>MVKLAEFSRTATFAWSHDKIPLLVSGTVSGTVDANFSTDSSLELWSLLAADSEKPIASLQVDSKFNDLDWSHNNKIIAGALDNGSLELYSTNEANNAINSMARFSNHSSSVKTVKFNAKQDNVLASGGNNGEIFIWDMNKCTESPSNYTPLTPGQSMSSVDEVISLAWNQSLAHVFASAGSSNFASIWDLKAKKEVIHLSYTSPNSGIKQQLSVVEWHPKNSTRVATATGSDNDPSILIWDLRNANTPLQTLNQGHQKGILSLDWCHQDEHLLLSSGRDNTVLLWNPESAEQLSQFPARGNWCFKTKFAPEAPDLFACASFDNKIEVQTLQNLTNTLDEQETETKQQESETDFWNNVSREESKEKPSVFHLQAPTWYGEPSPAAHWAFGGKLVQITPDGKGVSITNPKISGLESNTTLSEALKTKDFKPLINQRLVKVIDDVNEEDWNLLEKLSMDGTEEFLKEALAFDNDESDAQDDANNEKEDDGEEFFQQIETNFQPEGDFSLSGNIEQTISKNLVSGNIKSAVKNSLENDLLMEAMVIALDSNNERLKESVKNAYFAKYGSKSSLSRILYSISKREVDDLVENLDVSQWKFISKAIQNLYPNDIAQRNEMLIKLGDRLKENGHRQDSLTLYLAAGSLDKVASIWLSEFPDLEDKLKKDNKTIYEAHSECLTEFIERFTVFSNFINGSSTINNEQLIAKFLEFINLTTSTGNFELATEFLNSLPSDNEEVKTEKARVLIASGKSLPAQNPATATTSKAKYTNAKTNKNVPVLPTPGMPSTTSIPSMQAPFYGMTPGASANALPPKPYVPATTTSAPVHTEGKYAPPSQPSMASPFVNKTNSSTRLNSFAPPPNPYATATVPATNVSTTSIPQNTFAPIQPGMPIMGDYNAQSSSIPSQPPINAVSGQTPHLNRKANDGWNDLPLKVKEKPSRAKAVSVAPPNILSTPTPLNGIPANAASTMPPPPLSRAPSSVSMVSPPPLHKNSRVPSLVATSESPRASISNPYAPPQSSQQFPIGTISTANQTSNTAQVASSNPYAPPPQQRVATPLSGGVPPAPLPKASNPYAPTATTQPNGSSYPPTGPYTNNHTMTSPPPVFNKPPTGPPPISMKKRSNKLASIEQNPSQGATYPPTLSSSASPLQPSQPPTLASQVNTSAENVSHEIPADQQPIVDFLKEELARVTPLTPKEYSKQLKDCDKRLKILFYHLEKQDLLTQPTIDCLHDLVALMKEKKYKEAMVIHANIATNHAQEGGNWLTGVKRLIGIAEATLN[2x];> MVVIANAHNELIHDAVLDYYGKRLATCSSDKTIKIFEVEGETHKLIDTLTGHEGPVWRVDWAHPKFGTILASCSYDGKVLIWKEENGRWSQIAVHAVHSASVNSVQWAPHEYGPLLLVASSDGKVSVVEFKENGTTSPIIIDAHAIGVNSASWAPATIEEDGEHNGTKESRKFVTGGADNLVKIWKYNSDAQTYVLESTLEGHSDWVRDVAWSPTVLLRSYLASVSQDRTCIIWTQDNEQGPWKKTLLKEEKFPDVLWRASWSLSGNVLALSGGDNKVTLWKENLEGKWEPAGEVHQ;> MVVIANAHNEMIHDAVMDYYGKRMATCSSDKTIKIFEVEGETHKLIDTLTGHEGPVWRVDWAHPKFGTILASCSYDGKVMIWKEENGRWSQIAVHAVHSASVNSVQWAPHEYGPMLLVASSDGKVSVVEFKENGTTSPIIIDAHAIGVNSASWAPATIEEDGEHNGTKESRKFVTGGADNLVKIWKYNSDAQTYVLESTLEGHSDWVRDVAWSPTVLLRSYMASVSQDRTCIIWTQDNEQGPWKKTLLKEEKFPDVLWRASWSLSGNVLALSGGDNKVTLWKENLEGKWEPAGEVHQ

COPII mediates Endoplasmic Reticulum to Golgi trafficking of thousands of cargoes. ER export is mediated by the coat protein complex II (COPII), which minimally comprises five cytosolic proteins that form two concentric layers on the ER membrane—the inner and outer coat. The inner coat layer consists of the small GTPase Sar1 and the heterodimeric Sec23/24 complex, whilst the outer coat layer comprises the rod-shaped heterotetramer Sec13/31. Here we visualise the complete, membrane-assembled COPII coat by cryo-electron tomography and subtomogram averaging, revealing the full network of interactions within and between coat layers.

We next analysed rods that interconnect vertices in the right-handed direction. Surprisingly, in addition to the CTD appendages, a second region of ill-defined extra density was present near the Sec31 dimerisation region. Upon classification we could divide the right-handed rod dataset into two classes, both of which converged to resolutions between 13 and 15 Å. Analysis of the averages placed in the context of individual tomograms shows that the extra rods are sparsely and randomly distributed. We also discover a second interaction within the outer coat: in addition to the known interaction of Sec31 β-propellers with each other at vertices, these domains can also bind to the Sec31 dimerisation interface, at the centre of the α-solenoid region. This leads to extra outer coat rods creating a bridge between canonical rods. Occasionally these extra rods form a canonical vertex interaction at one end, and an orthogonal interaction with other rods at the other end. Such rods ‘glue’ mismatched patches of outer coat lattice together: they might therefore be important for outer coat stabilisation in a context of flexibility and adaptability. Due to limited particle numbers, the resolution we obtained does not allow us to precisely define the residues involved in the interaction between the β-propeller and the α-solenoid domains of Sec31.> GAMAKVQVNNVVVLDNPSPFYNPFQFEITFECIEDLSEDLEWKIIYVGSAESEEYDQVLDSVLVGPVPAGRHMFVFQADAPNPGLIPDADAVGVTVVLITCTYRGQEFIRVGYYVNNEYTETELRENPP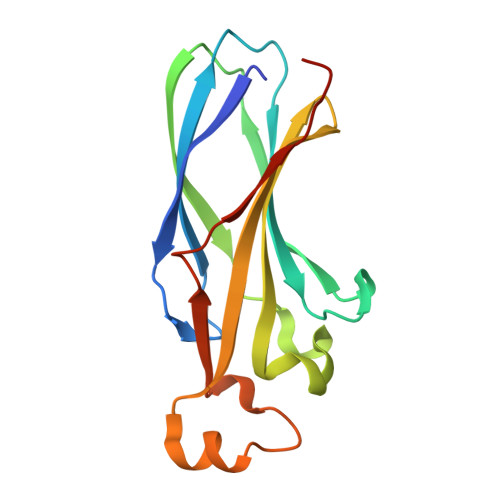VKPDFSKLQRNILASNPRVTRFHINWEDN>[4x]SLQKMKSSRKFLEGEPNIVIRKGELQYKVMKKNKIDINQLQSMLRQAGSFSIQEVEYAIMETNGMVSVLPKSDFDKPTNKDMQIPSKSVSLPITLIIDGEIVRDNLKEAGV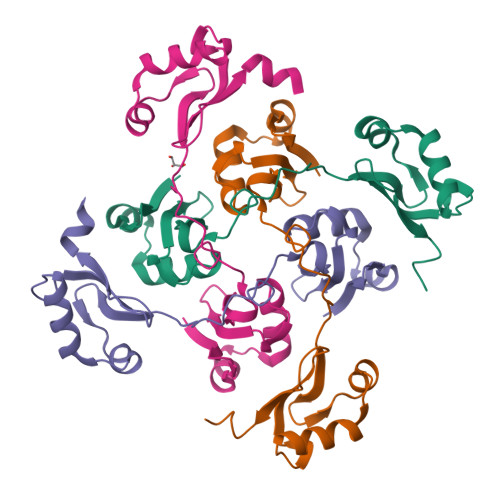DEQWLKQEMKKKNIDKTEDVLFAEWHKNKPLYTVTYEQSRST> MPFTIDSARGIFPNTLAADVVPATIARFSQLNAEDQLALIWFAYLEMGKTLTIAAPGAASMQLAENALKEIQAMGPLQQTQAMCDLANRADTPLCRTYASWSPNIKLGFWYRLGELMEQGFVAPIPAGYQLSANANAVLATIQGLESGQQITVLRNAVVDMGFTAGKDGKRIAEPVVPPQDTASRTKVSIEGVTNATVLNYMDNLNANDFDTLIELFTSDGALQPPFQRPIVGKENVLRFFREECQNLKLIPERGVTEPAEDGFTQ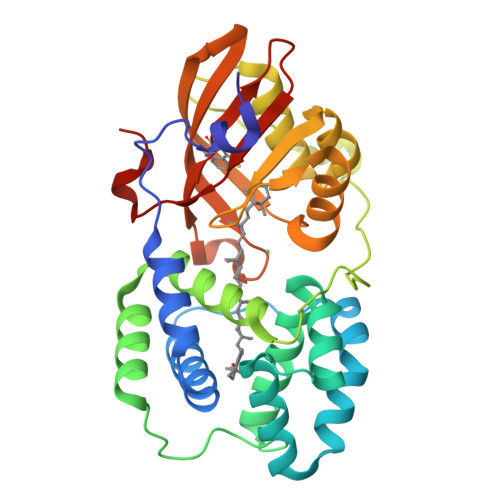IKVTGKVQTPWFGGNVGMNIAWRFLLNPEGKIFFVAIDLLASPKELLNFAR> SNAMPYTWKFLGISKQLSLENGIAKLNQLLNLEVDLDIQ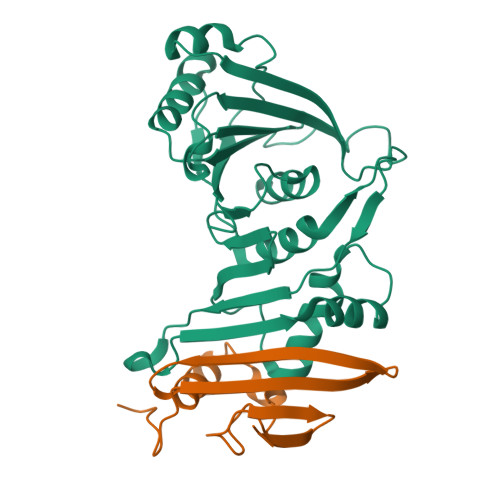TIRVPSDPDGGTAADEYIRYEMRLDISNLDEGTYSKFIFLGNSKMEVPMFLCYCGTDNRNEVVLQWLKAEYGVIMWPIKFEQKTMIKLADASIVHVTKENIEQITWFSSKLYFEPETQDKNLRQFSIEIPRESCEGLALGYGNTMHPYNDAIVPYIYNETGMAVERLPLTSVILAGHTKIMRESIVTSTRSLRNRVLAVVLQSIQF;> SNAGKKNEDSGEPVYISRYSSLVPIEKVGFTLKNEINSRIITIKLKFNGNDIFGGLHELCDKNLINIDKVPGWLAGENGSFSGTIMNGDFQREQVAKGGLL(1-hydroxyethane-1,1-diyl)bis(phosphonic 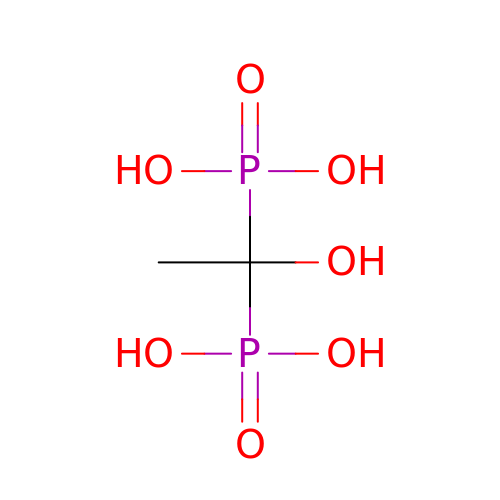acid) | C2 H8 O7 P2 | DBVJJBKOTRCVKF-UHFFFAOYSA-N>MGSSHHHHHHENLYFQGSQSAVSTLDRQMMGSALDNVQQINDMINTSISQKEDGTAYFSDWLTKDRYKPKNQSQITDKFTEYMKINKDVESIYTSDTEGHFTRYPDLQMPKGYNPIERDWYKKAVENKGKVVVT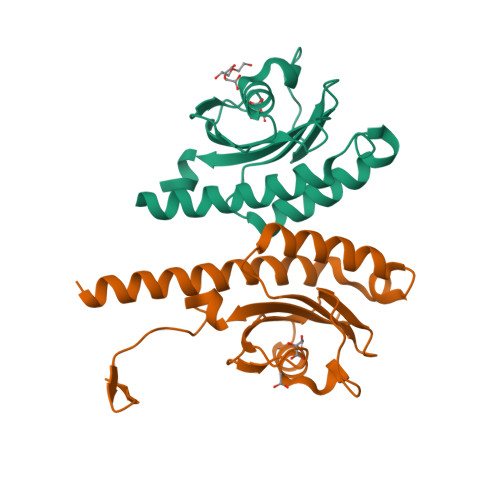DPYRTASTNTMVVTVVQQTKDGSGVVAINMKIDELLKTTKKVNIGKSGYAFILTKDKKVVAHPNRTSGTVL[2x]> AAPR;> IVGGYTCGANTVPYQVSLNSGYHFCGGSLINSQWVVSAAHCYKSGIQVRLGEDNINVVEGNEQFISASKSIVHPSYNSNTLNNDIMLIKLKSAASLNSRVASISLPTSCASAGTQCLISGWGNTKSSGTSYPDVLKCLKAPILSDSSCKSAYPGQITSNMFCAGYLEGGKDSCQGDSGGPVVCSGKLQG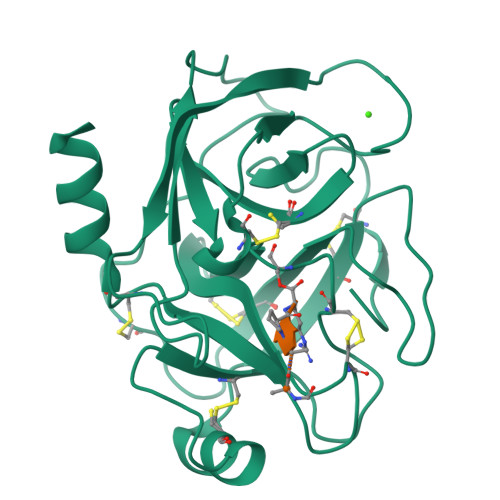IVSWGSGCAQKNKPGVYTKVCNYVSWIKQTIASN2-oxo-2-[(4-sulfamoylphenyl)amino]ethyl 7,8,9,10-tetrahydro-6H-cyclohepta[b]quinoline-11-carboxylate 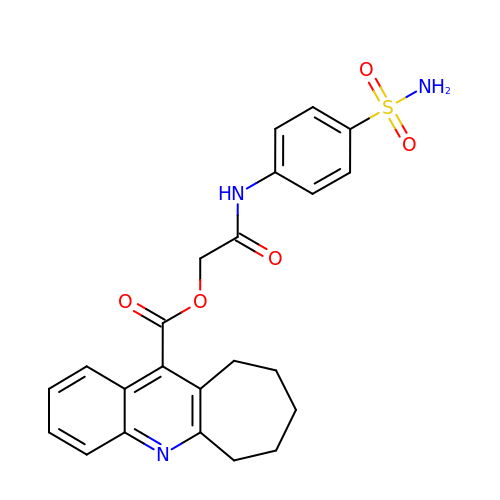| C23 H23 N3 O5 S | CZNAHALNBRNZRG-UHFFFAOYSA-N5-AMINO-5-DEOXY-1-O-PHOSPHONO-D-MANNITOL | C6 H16 N O8 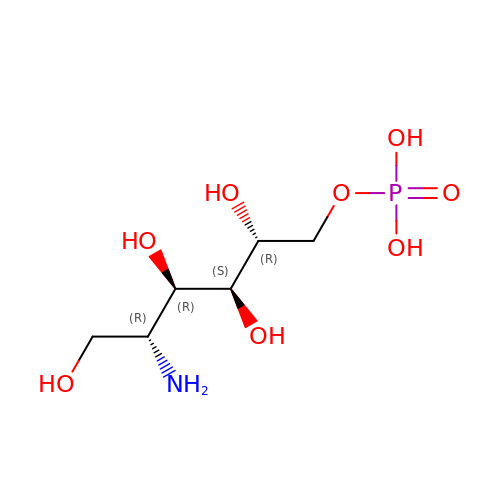P | LBNVXZROMBUNNQ-KVTDHHQDSA-N> PTTKVKLECNPTARIYRKHFLGKEHFNYYSLDTALGHLVFSLKYDVIGDQEHLRLLLRTKCRTYHDVIPISCLTEFPNVVQMAKLVCEDVNVDRFYPVLYPKASRLIVTFDEHVISNNFKFGVIYQKLGATSEEELFSTNEESPAFVEFLEFLGQKVKLQDFKGFRGGLDVTHGQTGTESVYCNFRNKEIMFHVSTKLPYTEGDAQQLQRKRHIGNDIVAVVFQDENTPFVPDMIASNFLHAYVVVQAEGGGPDGPLYKVSVTARDDVPFFGPPLPDPAVFRKGP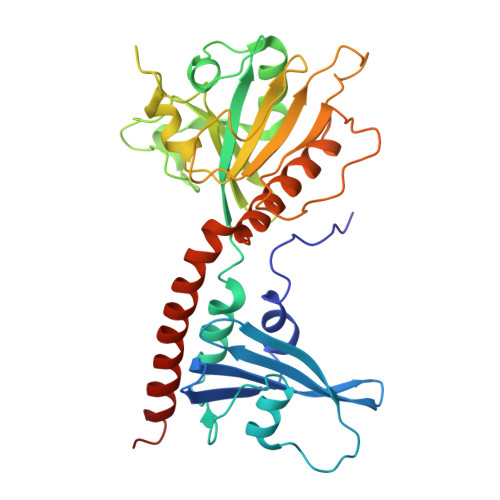EFQEFLLTKLINAEYACYKAEKFAKLEERTRAALLETLYEELHIHSQSMMGLGGDE> SLKRLAFSSLSHTLAPFPEGELDAHLSDADFTRVFTEEDDLDLVAQSLPLVLKVYEALHLQNPAHRGLSLAVGRLYIMYANAFVQTPAQYLPEDEFEAQNEAYSRARKLYLRGARYALSSLETAYPGFTREVFSGDEQRLHKVLSRCTRVDVGTLYWVGTGYVAAFALTPLGSALPDTVHAAVMMLERACDLWPSYQEGAVWNVLTKFYAAAPESF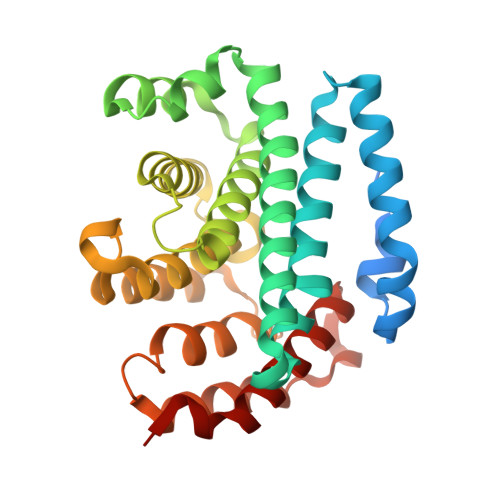GGGMEKAHTAFEHLTRYCSAHDPDHHITYADALCIPLNNRAGFDEALDRALAIDPESVPHNKLLVILSQKRARWLKAHVQDFFLD2-(5-fluoro-1H-indol-3-yl)ethan-1-amine | C10 H11 F N2 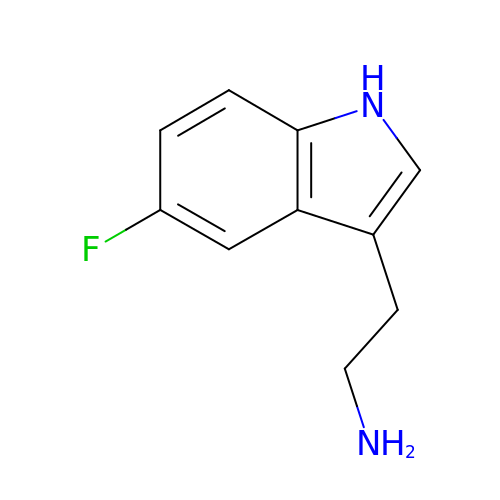| ZKIORVIXEWIOGB-UHFFFAOYSA-N4-[(phenylmethyl)amino]benzoic 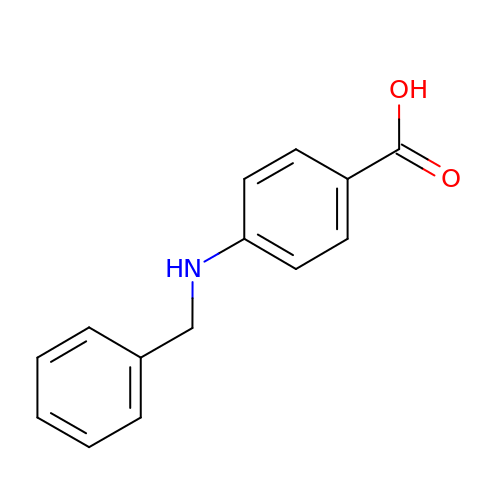acid | C14 H13 N O2 | NYNAMTQEBMCHNG-UHFFFAOYSA-N>AMPLDAGGQNSTQMVLAPGASIFRCRQC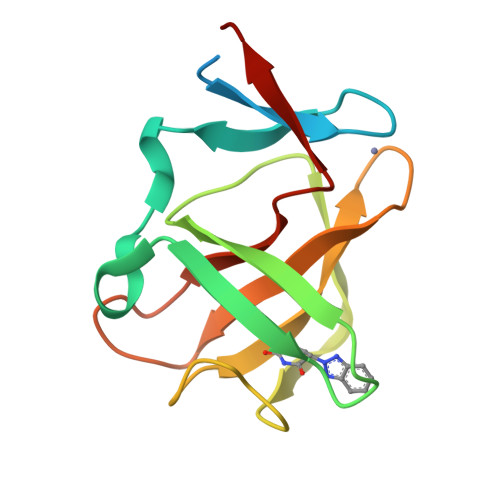GQTISRRDWLLPMGGDHEHVVFNPAGMIFRVWCFSLAQGLRLIGAPSGEFSWFKGYDWTIALCGQCGSHLGWHYEGGSQPQTFFGLIKDRLAEGPAD[3x]> MQLNNRDLKSIIDNEALAYAMYTVENRAIPNMIDGFKPVQRFVIARALDLARGNKDKFHKLASIAGGVADLGYHHGENSAQDAGALMANTWNNNFPLLDGQGNFGSRTVQKAAASRYIFARVSKNFYNVYKDTEYAPVHQDKEHIPPAFYLPIIPTVLLNGVSGIATGYATYILPHS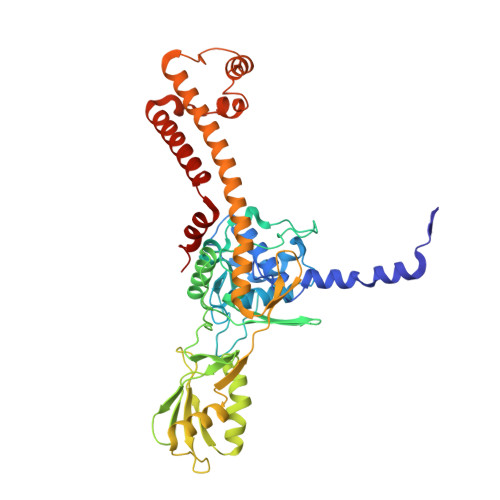VSSVKKAVLQALQGKKVTKPKVEFPEFRGEVVEIDGQYEIRGTYKFTSRTQMHITEIPYKYDRETYVSKILDPLENKGFITWDDACGEHGFGFKVKFRKEYSLSDNEEERHAKIMKDFGLIERRSQNITVINEKGKLQVYDNVVDLIKDFVEVRKTYVQKRIDNKIKETESAFRLAFAKAHFIKKVISGEIVVQGKTRKELTEELSKIDMYSSYVDKLVGMNIFHMTSDEAKKLAEEAKAKKEENEYWKTTDVVTEYTKDLEEIK>APQLHHHHHHDLYENLYFQGKLTTLDEADEAGKRIFGPRVGNELCEVKHVLDLCRIRESVSEELLQLEAKRQELNSEIAKLNLKIEACKKSIENAKQDLLQLKNVISQTEHSYKELMAQNQPKLSLPIRLLPEKDDAGLPPPKATRGCRLHNCFDYSRCPLTSGFPVYVYDSDQFVFGSYLDPLVKQAFQATARANVYVTENADIACLYVILVGEMQEPVVLRPAELEKQLYSLPHWRTDGHNHVIINLSRKSDTQNLLYNVSTGRAMVAQSTFYTVQYRPGFDLVVSPLVHAMSEPNFMEIPPQVPVKRKYLFTFQGEKIESLRSSLQEARSFEEEMEGDPPADYDDRIIATLKAVQDSKLDQVLVEFTCKNQPKPSLPTEWALCGEREDRLELLKLSTFALIITPGDPRLVISSGCATRLFEALEVGAVPVVLGEQVQLPYQDMLQWNEAALVVPKPRVTEVHFLLRSLSDSDLLAMRRQGRFLWETYFSTADSIFNTVLAMIRTRIQIPAAPIREEAAAEIPHRSGKAAGTDPNMADNGDLDLGPVETEPPYASPRYLRNFTLTVTDFYRSWNCAPGPFHLFPHTPFDPVLPSEAKFLGSGTGFRPIGGGAGGSGKEFQAALGGNVPREQFTVVMLTYEREEVLMNSLERLNGLPYLNKVVVVWNSPKLPSEDLLWPDIGVPIMVVRTEKNSLNNRFLPWNEIETEAILSIDDDAHLRHDEIMFGFRVWREARDRIVGFPGRYHAWDIPHQSWLYNSNYSCELSMVLTGAAFFHKYYAYLYSYVMPQAIRDMVDEYINCEDIAMNFLVSHITRKPPIKVTSRWTFRCPGCPQALSHDDSHFHERHKCINFFVKVYGYMPLLYTQFRVDSVLFKTRLPHDKTKCFKFI[2x]

Heparan sulfate is a highly modified O-linked glycan that performs diverse physiological roles in animal tissues. Though quickly modified, it is initially synthesised as a polysaccharide of alternating β-d-glucuronosyl and N-acetyl-α-d-glucosaminyl residues by exostosins. These enzymes generally possess two glycosyltransferase domains (GT47 and GT64)—each thought to add one type of monosaccharide unit to the backbone. The HS chain can be initiated from the tetrasaccharide linker by EXTL3 or (in some cases) by EXTL2, which add the first α-GlcNAc residue (GlcNAcT-I activity).

To gain further insight into the arrangement of these domains, we solved the structure of EXTL3ΔN by single-particle cryo-EM, producing a high-quality Coulomb potential map at 2.4 Å resolution. We then built and refined an ab initio model of the 170 kDa globular domain of an EXTL3 homodimer. In each chain, we were able to model two partial N-glycans at Asn592 and Asn790, respectively. The coiled coil domain, however, was not visible in the map, likely due to its flexibility with respect to the catalytic domain. Detailed analysis of the globular structure revealed that it is indeed composed of four glycosyltransferase-type domains, with one GT47 and GT64 domain provided by each chain. Within each chain, the GT47 and GT64 domains are connected by a linker region of 124 amino acids. Curiously, the N-terminal half of the linker region constitutes an extended loop that traverses 40 Å over the surface of the GT64 domain, forming a ‘cradle’. The GT64 domain and linker region appear to contribute the most to the homodimeric interaction (see Supplementary Table 4 for PISA35-calculated energy contributions), which appears to be stabilised by a pair of intermolecular disulfide bridges between Cys793 and Cys915 in the GT64 domain. Inspection of the structure revealed that the EXTL3 GT47 domain adopts a GT-B fold, with two distinct Rossman-fold subdomains. In spite of this sequence conservation, the GT47 domain of EXTL3 exhibits several unique features that point to a loss of activity in this particular enzyme. For instance, the side chains of Glu453 and Arg421 are engaged in a salt-bridge, which would direct Glu453 away from making interactions with the substrate. Moreover, our structural alignment revealed that, in contrast to other GT-B structures, the EXTL3 Cα4 helix exhibits an extra turn at its N-terminus that occludes a putative phosphate/donor sugar binding pocket.>[2x]MGQGNDTSEVMLLDTGWEFSQSGTEKWMPATVPGTVHQDLISHELLPNPFYGMNEKKIQWVENEDWEYRTSFIVSEEQLNRDGIQLIFEGLDTYADVYLNGSLLLKADNMFVGYTLPVKSVLRKGENHLYIYFHSPIRQTLPQYASNGFNYPADNDHHEKHLSVFSRKAPYSYGWDWGIRMVTSGVWRPVTLRFYDIATISDYYVRQLSLTDENARLSNELIVNQIVPQKIPAEVRVNVSLNGTTVTEVKQQVTLQPGINHITLPAEVTNPVRWMPNGWGTPTLYDFSAQIACGDRIVAEQSHRIGLRTIRVVNEKDKDGESFYFEVNGIPMFAKGANYIPQDALLPNVTTERYQTLFRDMKEANMNMVRIWGGGTYENNLFYDLADENGILVWQDFMFACTPYPSDPTFLKRVEAEAVYNIRRLRNHASLAMWCGNNEILEALKYWGFEKKFTPEVYQGLMHGYDKLFRELL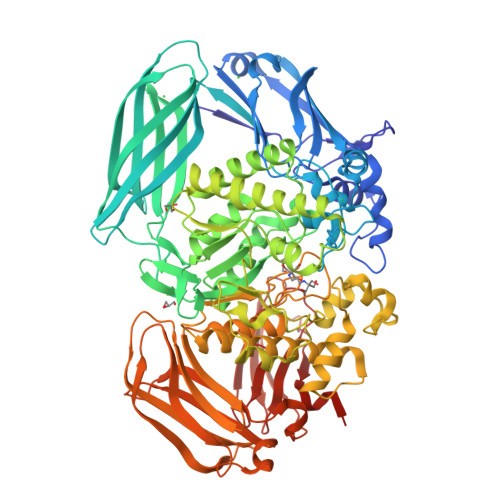PSTVKEFDSDRFYVHSSPYLANWGRPESWGTGDSHNWGVWYGKKPFESLDTDLPRFMSEFGFQSFPEMKTIAAFAAPEDYQIESEVMNAHQKSSIGNSLIRTYMERDYIIPESFEDFVYVGLVLQGQGMRHGLEAHRRNRPYCMGTLYWQLNDSWPVVSWSSIDYYGNWKALHYQAKRAFAPVLINPIQQNDSLSVYLISDRLDTMEQMTLEMKVVDFDGKTLGKKIQVHSLEVPANTSKCVYRAKLDGWLTPEDCRRSFLKLILKDKSGHQVAESVHFFRKTKDLQLPPTSVSYQMKQTDGKCELTLFSSMLAKDIFIETPLQGARYSDNFFDLLPGERKKVIITSPRIKKGEELPVNIKHIRETYKEHHHHHH>[2x]VYRRLVSGTEGEKDFRVLLSKKSGERLSPWHDIPLFPNGRDARPLLFNMVVEIPKNTRRKMEMQLRLPFTPIMQDLKKDGSLREYAS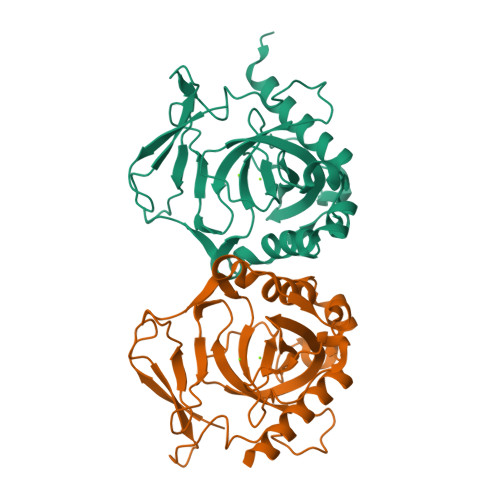TLYWNYGAFPQTWEDPREPGGREVFHARGDGDPLDVVEIGSEVLPVGGVVPVKVLGALAMIDGGELDWKVLAIREGDPLFSQLNSVADVERLCRGVVPGIREWFRWYKLPTDNVVNQFGHDEAALPAADAERVVYRAHEHYLRLLSEE> PLPWCPHLVAVCPIPAAGLDVTQPCGDCGTIQENWVCLSCYQVYCGRYINGHMLQHHGNSGHPLVLSYIDLSAWCYYCQAYVHHQALLDVKN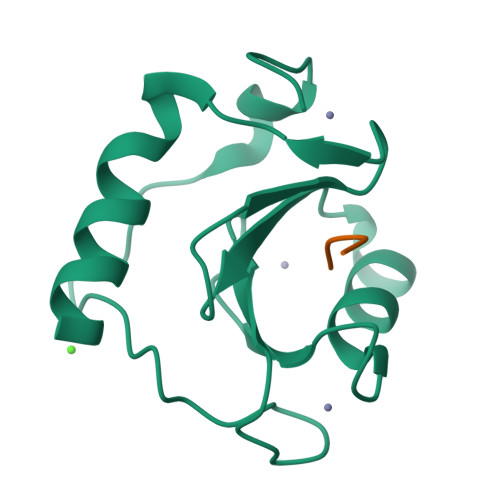IAHQNKFGEDMPHPH;> RLRGG Many components, including pili and polysaccharides, are essential for the formation of these biofilms, but the octaheme c-type cytochrome OmcZ is the only cytochrome out of over 80 multiheme proteins in the Geobacter sulfurreducens genome necessary for long-distance conductivity in electrode associated biofilms. The omcZ gene is upregulated 400–800% in conductive electrode biofilms, producing a 50 kDa periplasmic preprotein that is processed by the OzpA protease to a 30 kDa octaheme form. OmcZ represents one of three multiheme cytochrome filaments identified to date, along with the proteins OmcS and OmcE. In conductive-probe AFM measurements of enriched filaments cast on gold surfaces, OmcZ can demonstrate up to 1000-fold higher conductivity than preparations primarily consisting of OmcS, indicating that internal packing or external accessibility of hemes may be uniquely suited for interfacing OmcZ with electrodes.

In this work, we describe the cryo-EM structure of G. sulfurreducens OmcZ, and show that it forms a multiheme cytochrome nanowire different from OmcS and OmcE in both protein fold and heme arrangement. OmcZ filaments are ~50 Å at their widest point and coordinate eight heme molecules per cytochrome subunit. Using the AlphaFold prediction as a starting model and iterative model refinements, residues P27 to S284 could fit into the map, with the signal peptide (residues 1–26) and the C-terminal Ig-domains missing. For all eight hemes per OmcZ subunit, two histidines axially coordinate iron at the center of each heme, and the vinyl groups of each heme form covalent thioether bonds with cysteines. All hemes in OmcZ are thus close to two other hemes, with the exception of heme 6 which is only close to one other heme, heme 5, at an edge-to-edge distance of 4.6 Å. In OmcZ, all eight hemes are coordinated by histidines within the same subunit. Also unique to OmcZ is the motif binding heme 1, which lies at the N-terminal interface. Instead of the canonical CxxCH motif, additional amino acids form a 14-residue loop between C77 and C92 (rather than the expected pattern of C89, C92, and H93). In OmcZ, heme 6 is largely solvent-exposed in every subunit in the filament. In contrast, the OmcZ solvent-exposed heme raises the possibility that networks of OmcZ filaments may form with a multiplicity of paths through which electrons can flow, supporting a more conductive biofilm.

> MKKKVLIGASLAAVVLTGAAMVGAAVPPPPVNQFLGIYDTKFPNLTKADCLECHVSDTVLVQQHHALINTVTPPASCINTSGTVPPTLATGCHVMVPDGSGGFTFQDFRNCFNCHTQTPHHTSPAAVAKDCKYCHGNFIDNPLDGHYIPTYSASSVTPMPSGRSVTATDGNVVIVQGCEACHQAAPNAIDPKTNTVRPIFSNQDTHHGTGITDCNLCHNTSSNVPIRQCEVCHGVNSLHNIQKDSPNAANLGTVKPGLEDLGWGHIGNNWDCQGCHWSWFGNSSPYTNATVPAINGQSSYTVTAGKEAVLTIVGSSFVNVGPDGVTTYQPTVALVSGSTSLTLTPFSVTESEIKVSVPALVEGVYELRITKANKVSNLAKLTVAPARIIASATLATGKTLTITGTGFGPAPSSEYDAGIGVYAGTTQANVISWSDTKVVATSPDFATNGYVTVKTINGPLSGKILAAPKKVKR> SAFEVGRNVAVTEGAVVFENEYFQLLQYKPLTDKVHARPLLM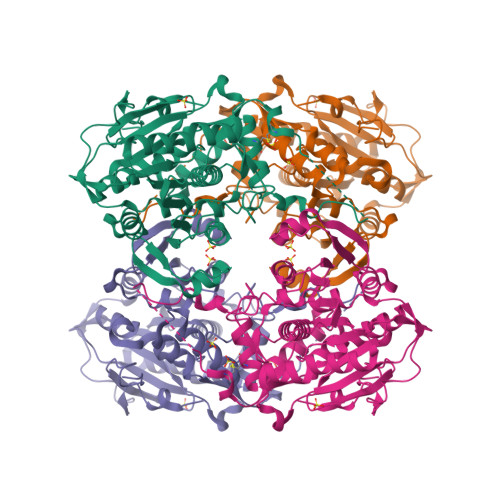VPPCINKYYILDLQPESSLVRHVVEQGHTVFLVSWRNPDASMAGSTWDDYIEHAAIRAIEVARDISGQDKINVLGFAVGGTIVSTALAVLAARGEHPAASVTLLTTLLDFADTGILDVFVDEGHVQLREATLGGGAGAPCALLRGLELANTFSFLRPNDLVWNYVVDNYLKGNTPVPFDLLFWNGDATNLPGPWYCWYLRHTYLQNELKVPGKLTVCGVPVDLASIDVPTYIYGSREDHIVPWTAAYASTALLANKLRFVLGASGHIAGVINPPAKNKRSHWTNDALPESPQQWLAGAIEHHGSWWPDWTAWLAGQAGAKRAAPANYGNARYRAIEPAPGRYVKAKA>SAAATQAVPAPNQQPEVFCNQIFINNEWHDAVSRKTFPTVNPSTGEVICQVAEGDKEDVDKAVKAARAAFQLGSPWRRMDASHRGRLLNRLADLIERDRTYLAALETLDNGKPYVISYLVDLDMVLKCLRYYAGWADKYHGKTIPIDGDFFSYTRHEPVGVCGQIIPWNFPLLMQAWKLGPALATGNVVVMKVAEQTPLTALYVANLIKEAGFPPGVVNIVPGFGPTAGAAIASHEDVDKVAFTGSTEIGRVIQVAAGSSNLKRVTLQLGGKSPNIIMSDADMDWAVEQAHFALFFNQGQSCSAGSRTFVQEDIYDEFVERSVARAKSRVVGNPFDSKTEQGPQVDETQFKKILGYINTGKQEGAKLLCGGGIAADRGYFIQPTVFGDVQDGMTIAKEEIFGPVMQILKFKTIEEVVGRANNSTYGLAAAVFTKDLDKA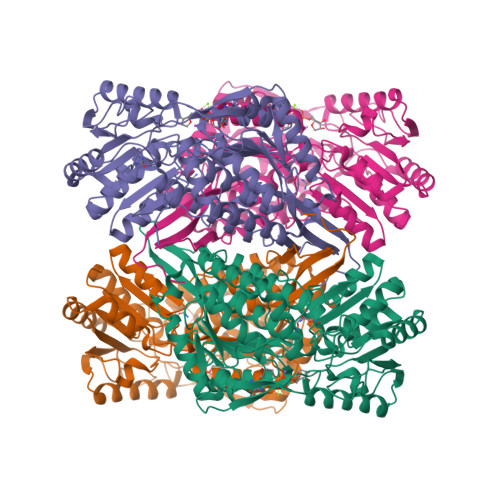NYLSQALQAGTVWVNCYDVFGAQSPFGGYKMSGSGRELGEYGLQAYTEVKTVTVKVPQKNS[8x]> MASNFTQFVLVDNGGTGDVTVAPSNFANGVAEWISSNSRSQAYKVTCSVRQSSAQNRKYTIKVEVPKVATQTVGGV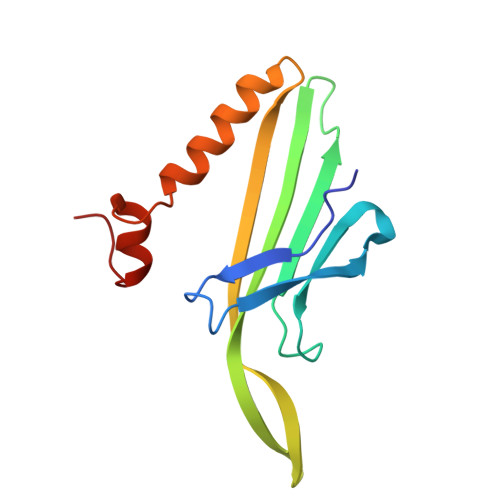ELPVAAWRSYLNMELTIPIFATNSDCELIVKAMQGLLKDGNPIPSAIAANSGIY>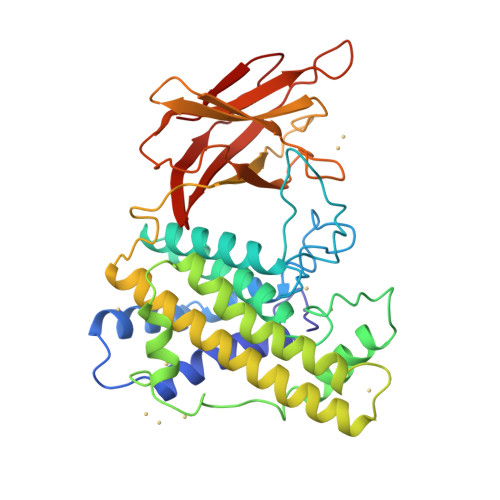 WDGKIDGTGTHAMIVTQGVSILENDLSKNEPESVRKNLEILKENMHELQLGSTYPDYDKNAYDLYQDHFWDPDTDNNFSKDNSWYLAYSIPDTGESQIRKFSALARYEWQRGNYKQATFYLGEAMHYFGDIDTPYHPANVTAVDSAGHVKFETFAEERKEQYKINTVGCKTNEDFYADILKNKDFNAWSKEYARGFAKTGKSIYYSHASMSHSWDDWDYAAKVTLANSQKGTAGYIYRFLHDVSEGNDPSVGKNVKELVAYISTSGEKDAGTDDYMYFGIKTKDGKTQEWEMDNPGNDFMTGSKDTYTFKLKDENLKIDDIQNMWIRKRKYTAFPDAYKPENIKVIANGKVVVDKDINEWISGNSTYNIK> MASMKKSTENESTNYQYKIQELRKLLKSLLLNYLELIGVLSINPDMYERKVENIRTILVNIHHLLNEYRP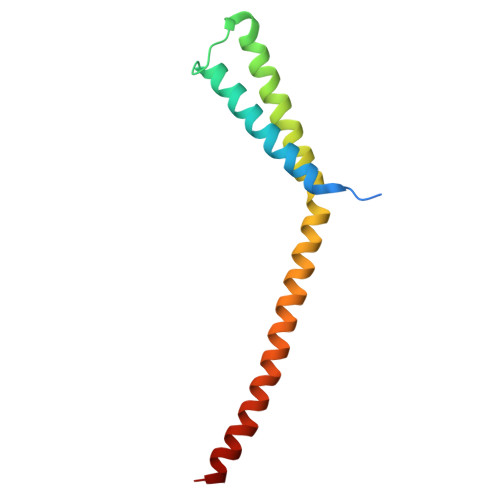HQSRESLIMLLEEQLEYKRGEIREIEQVCKQVHDKLTS>QDMVSPPPPIADEPLTVNTGIYLIECYSLDDKAETFKVNAFLSLSWKDRRLAFDPVRSGVRVKTYEPEAIWIPEIRFVNVENARDADVVDISVSPDGTVQYLERFSARVLSPLDFRRYPFDSQTLHIYLIVRSVDTRNIVLAVDLEKVGKNDDVFLTGWDIESFTAVVKPANFALEDRLESKLDYQLRISRQYFSYIPNIILPMLFILFISWTAFWSTSYEANVTLVVSTLIAHIAFNILVETNLPKTPY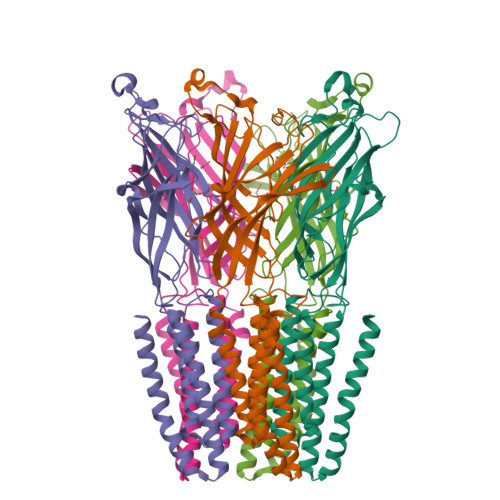MTYTGAIIFMIYLFYFVAVIEVTVQHYLKVESQPARAASITRASRIAFPVVFLLANIILAFLFFGF[5x]>[4x]GMGDVMDTSKAVIQRFNR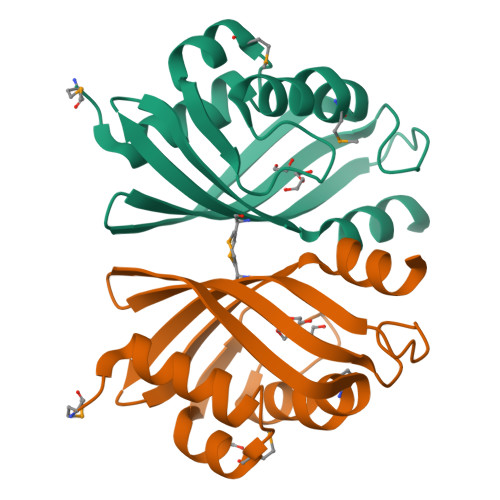EVIENGDMAAFAELVAPDFVNHSAPPGVSPGPDGFAGFFTGMLHPALSDIRVHIHEQIEENGKVVTRKTIEATHTGAFFGQPASGKRIAIHAMDIVVVRDGKYAEHWSCADLYGALAQIRAA> SQRKPRKLGQIKVLDGEDQYYKCLSPGACAPEE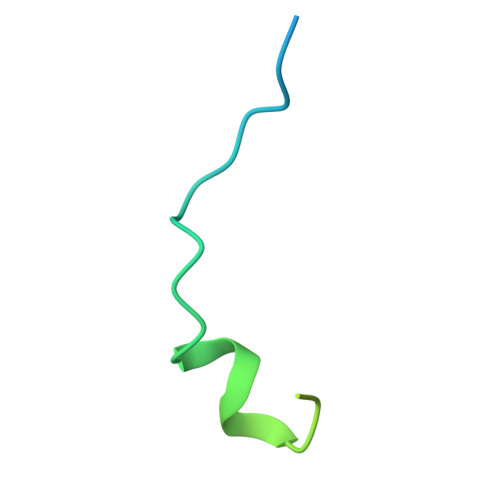THSVHPFFFSSSPREDPFAQH Here, inspired by natural and re-engineered protein–peptide systems, we set out to design proteins made out of repeating units that bind peptides with repeating sequences, with a one-to-one correspondence between the repeat units of the protein and those of the peptide. We use geometric hashing to identify protein backbones and peptide-docking arrangements that are compatible with bidentate hydrogen bonds between the side chains of the protein and the peptide backbone. We design repeat proteins to bind to six different tripeptide-repeat sequences in polyproline II conformations. The proteins are hyperstable and bind to four to six tandem repeats of their tripeptide targets with nanomolar to picomolar affinities in vitro and in living cells.

Reasoning that proline-containing peptides would incur a lower entropic cost upon binding than non-proline-containing peptides, we decided to start our experimental characterization with designs containing at least one proline residue; in most of these designs, the peptide backbone is in or near the polyproline II portion of the Ramachandran map. For the polyproline helix, there are roughly three residues per turn, and, probably because of this, we obtained more designs that target three-residue than two-residue proline-containing repeat units. Crystal structures reveal repeating interactions between protein and peptide interactions as designed, including ladders of hydrogen bonds from protein side chains to peptide backbones. Our results show that by matching superhelical parameters between repeating-protein and repeating-peptide conformations, and incorporating specific hydrogen-bonding and hydrophobic interactions between matched protein and peptide repeats, we can now design modular proteins that bind to extended peptides with high affinity and specificity.

> MDEEREKLKEKLKEVLRRAKEAKKKGDKEKLIELAYEAAALAAWIIHKDSNDDEIVELAKEALKLVLEAAKEAKKNGDKEKLIKLAYLAAAVAAWIIHTDGDDDEIVELAKEALKLVLEAAKEAKKNGDKEKLIKLAYLAAAVAAWIITTDGDDDEIVELAKEALKLVLEAAKEAKKNGDKEKLIKLAYLAAAVAAWIIHTDGDDDEIVELAKEALKLVLEAAKEAKKNGDKEKLIKLAYLAAAVAAWIITTDGDDEEIVELAKEALKLVKEAAEEAEKQGDEELREKLRYLSEAVREWIERND;> PLPPLPPLPPLPPLPPLPP> MWHSSLRYVSFKRLPFGRRSTSGGVNFNKGLLTDRERGDPFTEPHAYRNKKSIAAISKVAKKQDILLREEKQRKELDKIQSGYVTERELHIGCDKPLGGNANEIARVIDEQALISPTPGEKCSTALRELMENEVDRRNHMMDKFGQPVGAREFHRLFKELRHADNEAETIERHQTRLVEEYGVYPSLRLDAYMLDDDTYFPEWVNALPYSIRDRVKFGSLGLTEKDEALRVTLGRMPLDRRRREWERLKKAKEYKAAKEETLTLAELRDARQGKRRFHWLQRKRQKRASILRRLALRKPDAFELWPSRVVDYSQRIAFIAQHVENGLDTKGQWPLDPEELARARVRRSKEEAERTFLMSAEEKRAHKKLSGRSGDGSISEMLQSLEVPDKPFKRLSRKVYAN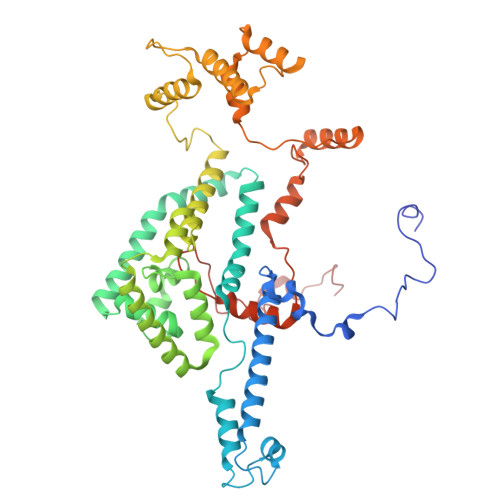RVNAIVHGDQDEYGRRYRKMETRSKRRMRPYASLGEIGLENELRKEPRINAKGLNNTDDEDWPRHTKSWGDGMPSMRYGS> GSIPGLERALQQYTLEPSEKPFDLKSVPLATAPLAEQRTESTPVTAAKQPEKVAATRQEIFQEQLAAVPEFQGLGPLFKSSPEPVALTESETEYVIRCTKHTFTDHMVFQFDCTNTLNDQTLENVTVQMEPSEAYEVLCYVPARSLPYNQPGTCYTLVALPKEDPTAVACTFSCVMKFTVKDCDPTTGEADDEGYEDEYVLEDLEVTIADHIQKVMKLNFEAAWDEVGDEFQKEETFTLSTIKTLEEAVGNIVKF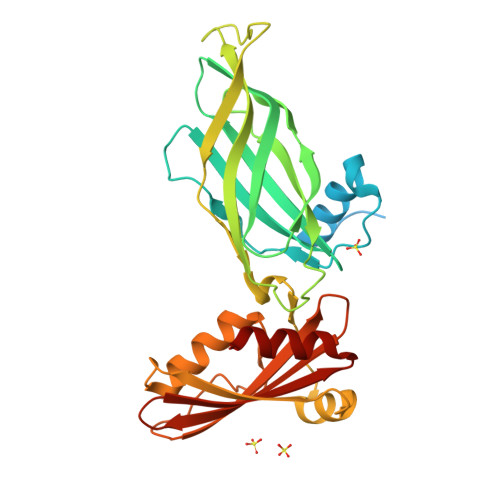LGMHPCERSDKVPDNKNTHTLLLAGVFRGGHDILVRSRLLLLDTVTMQVTARSSEELPVDIVLASVG> XVALDPFDFSIVLNKIKSQLEESKEWIRRSNKIL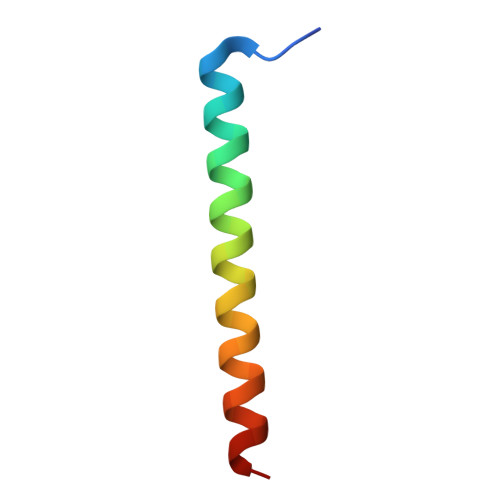DSIX>[4x]MTGNLVTKNSLTPDVRNGIDFKIADLSLADFGRKELRIAEHEMPGLMSLRREYAEVQPLKGARISGSLHMTVQTAVLIETLT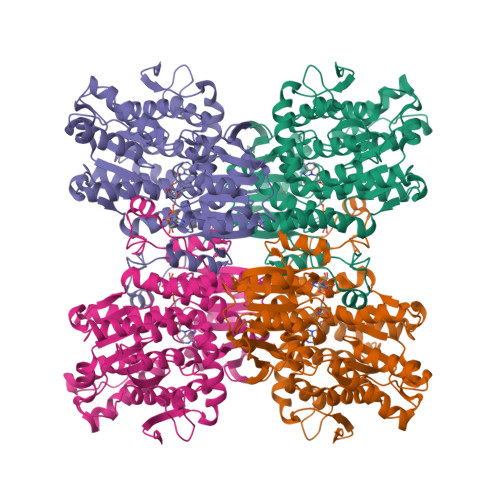ALGAEVRWASCNIFSTQDHAAAAVVVGPHGTPDEPKGVPVFAWKGETLEEYWWAAEQMLTWPDPDKPANMILDDGGDATMLVLRGMQYEKAGVVPPAEEDDPAEWKVFLNLLRTRFETDKDKWTKIAESVKGVTEETTTGVLRLYQFAAAGDLAFPAINVNDSVTKSKFDNKYGTRHSLIDGINRGTDALIGGKKVLICGYGDVGKGCAEAMKGQGARVSVTEIDPINALQAMMEGFDVVTVEEAIGDADIVVTATGNKDIIMLEHIKAMKDHAILGNIGHFDNEIDMAGLERSGATRVNVKPQVDLWTFGDTGRSIIVLSEGRLLNLGNATGHPSFVMSNSFANQTIAQIELWTKNDEYDNEVYRLPKHLDEKVARIHVEALGGHLTKLTKEQAEYLGVDVEGPYKPDHYRY>[2x]MRDYADNDSILLKHGWCEMLKGGVIMDVKNVEQAKIAEKAGAIGVMILENIPSELRNTDGVARSVDPLKIEEIRKCISINVLAKVRIGHFVEAQILEELKVDMLDESEVLTMADEYNHINKHKFKTPFVCGCTNLGEALRRISEGASMIRTKGEAGTGNIIEAIK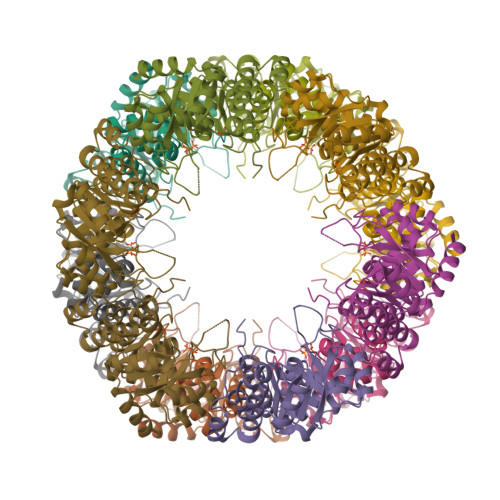HIRTVNNEIKYLCSLDESEVYNFAKKLRAPIDLILLTRKLKRLPVVNFAAGGIATPADAAMCMQLGMDGVFVGSGIFESENPQKMASSIVMAVSNFNNPKILLNVSLGLGKAMHGNTKVSNKWKNKSEEDNS>MRGSHHHHHHGSLSSSPSEILQELGKGSTHPQPGVSPPAAPAAPGPKDGPGETDAFGNSEGKELVASGENKIKQGLLPSLEDLLFYTIAEGQEKIPVHKFITALKSTGLRTSDPRLKECMDMLRLTLQTTSDGVMLDKDLFKKCVQSNIVLLTQAFRRKFVIPDFMS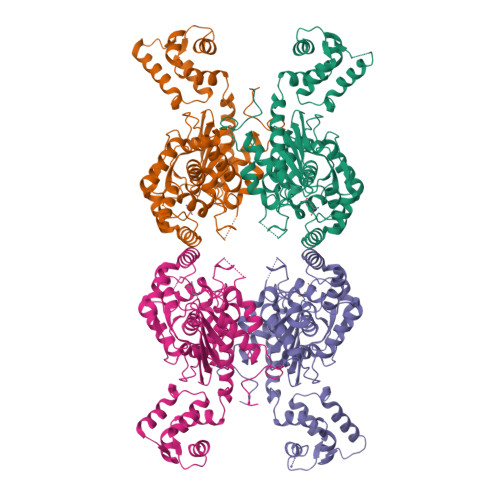FTSHIDELYESAKKQSGGKVADYIPQLAKFSPDLWGVSVCTVDGQRHSTGDTKVPFCLQSCVKPLKYAIAVNDLGTEYVHRYVGKEPSGLRFNKLFLNEDDKPHNPMVNAGAIVVTSLIKQGVNNAEKFDYVMQFLNKMAGNEYVGFSNATFQSERESGDRNFAIGYYLKEKKCFPEGTDMVGILDFYFQLCSIEVTCESASVMAATLANGGFCPITGERVLSPEAVRNTLSLMHSCGMWDFSGQFAFHVGLPAKSGVAGGILLVVPNVMGMMCWSPPLDKMGNSVKGIHFCHDLVSLCNFHNYDNLRHFAKKLDPRREGGDQRHSFGPLDYESLQQELALKETVWKKVSPESNEDISTTVVYRMESLGEKS[4x]> SRLNRESVIDAALELLNETGIDGLTTRKLAQKLGIEQPTLYWHVKNKRALLDALAVEILARHHDYSLPAAGESWQSFLRNNAMSFRRALLRYRDGAKVALGTRPDEKQYDTVETQLR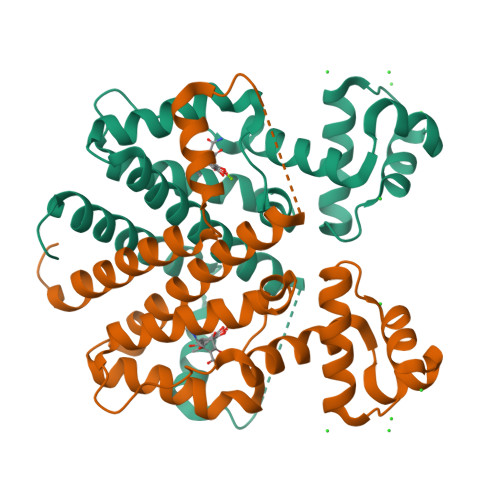FMTENGFSLRDGLYAISAVSHFTLGAVLEQQEHTAALTDRPAAPDENLPPLLREALQIMDSDDGEQAFLHGLESLIRGFEVQLTALLQIV>MIPVTELRYFADTQPAYRILKPWWDVFTDYISIVMLMIAVFGGTLQVTQDKMICLPCKWVTKDSCNDSFRGWAAPGPEPTYPNSTILPTPDTGPTGIKYDLDRHQYNYVDAVCYENRLHWFAKYFPYLVLLHTLIFLACSNFWFKFPRTSSKLEHFVSILLKCFDSPWTTRALSETVVEESDPKPAFSKMNGSMDKKSSTVSEDVEATVPMLQRTKSRIEQGIVDRSETGVLDKKEGEQAKALFEKVKKFRTHVEEGDIVYRLYMRQTIIKVIKFILIICYTVYYVHNIKFDVDCTVDIESLTGYRTYRCAHPLATLFKILASFYISLVIFYGLICMYTLWWMLRRSLKKYSFESIREESSYSDIPDVKNDFAFMLHLIDQYDPLYSKRFAVFLSEVSENKLRQLNLNNEWTLDKLRQRLTKNAQDKLELHLFMLSGIPDTVFDLVELEVLKLELIPDVTIPPSIAQLTGLKELWLYHTAAKIEAPALAFLRENLRALHIKFTDIKEIPLWIYSLKTLEELHLTGNLSAENNRYIVIDGLRELKRLKVLRLKSNLSKLPQVVTDVGVHLQKLSINNEGTKLIVLNSLKKMANLTELELIRCDLERIPHSIFSLHNLQEIDLKDNNLKTIEEIISFQHLHRLTCLKLWYNHIAYIPIQIGNLTNLERLYLNRNKIEKIPTQLFYCRKLRYLDLSHNNLTFLPADIGLLQNLQNLAITANRIETLPPELFQCRKLRALHLGNNVLQSLPSRVGELTNLTQIELRGNRLECLPVELGECPLLKRSGLVVEEDLFNTLPPEVKERLWRADKEQA[6x]

VRAC is a ubiquitously expressed mammalian anion channel implicated in diverse physiological processes including volume regulation, cell proliferation, release of excitatory amino acids, and apoptosis. Previous studies have shown that SWELL1 is required for VRAC activity, and that the presence of other LRRC8 subunits dictates functional characteristics of VRAC, including pore properties. SWELL1 is organized as a hexameric trimer of dimers with a four-layer domain architecture and an overall jellyfish-like shape. The transmembrane (TM) and extracellular domains (ECDs) surround the central pore axis, and share a previously unappreciated structural homology with the connexin and innexin gap junction channels.

To produce homomeric SWELL1, human SWELL1-FLAG was recombinantly expressed in LRRC8(B,C,D,E)-/- HEK293-F suspension cells, then solubilized in 1% decyl maltose neopentyl glycol (DMNG) detergent, followed by purification and exchange into 0.05% digitonin for structure determination by cryo-EM. Image analysis and reconstruction yielded a ~4 Å resolution map that was used to build a molecular model of SWELL1 (Figure 1—figure supplements 3–4). The ECDs, TMs, and ILDs all share the same 6-fold symmetric arrangement; however, in the cytosol, LRR domains dimerize in a parallel fashion with each LRR at either a 10 or −20° offset relative to the rest of its protomer, producing a 3-fold symmetric trimer of dimers. The nonequivalence between identical subunits arises from a hinge around the conserved residue L402 in a helix of the TM4-LRR linker (Figure 2D and Figure 1—Figure supplements 6 and 7). In the extracellular domain, 25 Å above the membrane, a ring of arginines (R103) at the N-terminal tip of the extracellular helix forms the narrowest constriction in the channel structure. Therefore, R103 is a critical residue within SWELL1 that impacts ion selectivity as well as pore block of heteromeric VRAC channels. Within the pore, constrictions are observed at pore-facing residues T44 and T48. Near the bottom of the pore cavity, a constriction at the intracellular face of the membrane corresponds to a short N-terminal coil (NTC) sitting parallel to the inner leaflet of the membrane. The first 14 residues of the N-terminus of the channel are not resolved in the cryo-EM density, presumably due to flexibility.(3S)-2-fluoro-3,7-dimethylocta-1,6-dien-3-yl trihydrogen diphosphate | C10 H19 F 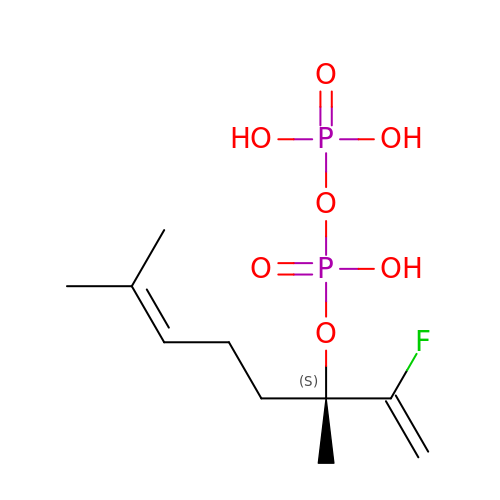O7 P2 | UEWCETXFDYIXPA-JTQLQIEISA-N> HWKTRAVPGAGTFGSAVAGQELPLCGVRAYYPPNAYIPAQVRDWLEFAHRPGLMATVPWTMADEPAERLGIFPVSPS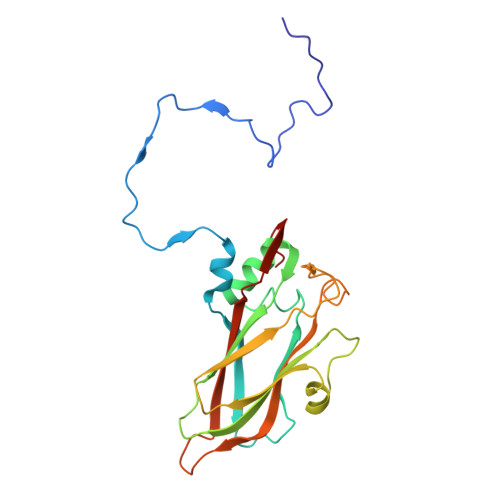AIAGTGAPISYVISLFSQWRGELAAHLLFTGSAQHYGRLVVCYTPAAPQPPSTMQEAMRGTYTVWDVNAASTLEFTIPFISNSYWKTVDVNNPDALLSTTGYVSIWVQNPLVGPHTAPASALVQAFISAGESFNVRLMQNPALTSQ Ataxia-telangiectasia mutated (ATM) is a large protein kinase with a central role in the cellular response to DNA double-strand breaks (DSBs) and related genotoxic stress. ATM, which belongs to the phosphatidylinositol 3-kinase-like protein kinase (PIKK) family, is essential for the sensing of DSBs during the cell cycle. MRN contributes to the localization of ATM to DSBs, and together with double-stranded DNA (dsDNA), it activates ATM as a protein kinase.

As the Nbs1 C-terminal half is unstructured or loosely folded, we made cryo-EM grids using a 28-residue peptide (207 μM) that encompasses the acidic region and FxF/Y motif of human Nbs1 (residues 727–754, hereafter referred to as Nc28) and human ATM (1.2 μM). After focused refinements of the ATM Spiral domain, we built a 10-residue Nbs1 segment (740ADDLFRYNPY749) into the improved density guided by the unambiguous density of the side chains for Phe744 and Tyr746. The Nbs1 peptide adopts an overall extended conformation except for one turn of a 310 helix in the middle (residues Asp742 to Arg745). It binds to a hydrophobic groove between two helical repeats formed by helices sα39 to sα42 (denoted ‘s’ for Spiral domain helices). Phe744 inserts deepest into the hydrophobic groove and makes van der Waals contacts to the side chains of Ser978, Arg981, Cys987, Val1021, Ala1024, Phe1025, Leu1028, and Tyr1034 of ATM. Of the two acidic residues that precede the Leu743-Phe744 pair, Asp741 hydrogen bonds with Ser978 and Arg981, while Asp742 is solvent exposed and uninvolved in ATM contacts. Tyr746 is the last Nbs1 residue that contacts ATM. Its side chain, which is stabilized by intramolecular stacking with Pro748, packs with side chain and backbone groups of Gly1016, Gln1017, and Thr1020 of ATM. The ATM structural elements at the Nbs1 binding site, including the hydrophobic pocket and adjacent cleft, are nearly identical in both the apo and Nc28-bound structures, indicating that Nc28 binding does not induce any noticeable structural rearrangements to this region. Additionally, no significant changes to the structure of the kinase domain were observed when comparing the unbound and Nc28-bound states. F744A and FRY to AAA mutations appeared to disrupt the interaction almost completely, whereas Y746A showed an intermediate effect. These results indicate that Nbs1 Phe744 is central to ATM binding, Tyr746 clearly contributes, while Arg745 makes at most a minor contribution in our assay.

>[2x]MSLVLNDLLICCRQLEHDRATERKKEVEKFKRLIRDPETIKHLDRHSDSKQGKYLNWDAVFRFLQKYIQKETECLRIAKPNVSASTQASRQKKMQEISSLVKYFIKCANRRAPRLKCQELLNYIMDTVKDSSNGAIYGADCSNILLKDILSVRKYWCEISQQQWLELFSVYFRLYLKPSQDVHRVLVARIIHAVTKGCCSQTDGLNSKFLDFFSKAIQCARQEKSSSGLNHILAALTIFLKTLAVNFRIRVCELGDEILPTLLYIWTQHRLNDSLKEVIIELFQLQIYIHHPKGAKTQEKGAYESTKWRSILYNLYDLLVNEISHIGSRGKYSSGFRNIAVKENLIELMADICHQVFNEDTRSLEISQSYTTTQRESSDYSVPCKRKKIELGWEVIKDHLQKSQNDFDLVPWLQIATQLISKYPASLPNCELSPLLMILSQLLPQQRHGERTPYVLRCLTEVALCQDKRSNLESSQKSDLLKLWNKIWCITFRGISSEQIQAENFGLLGAIIQGSLVEVDREFWKLFTGSACRPSCPAVCCLTLALTTSIVPGTVKMGIEQNMCEVNRSFSLKESIMKWLLFYQLEGDLENSTEVPPILHSNFPHLVLEKILVSLTMKNCKAAMNFFQSVPECEHHQKDKEELSFSEVEELFLQTTFDKMDFLTIVRECGIEKHQSSIGFSVHQNLKESLDRCLLGLSEQLLNNYSSEITNSETLVRCSRLLVGVLGCYCYMGVIAEEEAYKSELFQKAKSLMQCAGESITLFKNKTNEEFRIGSLRNMMQLCTRCLSNCTKKSPNKIASGFFLRLLTSKLMNDIADICKSLASFIKKPFDRGEVESMEDDTNGNLMEVEDQSSMNLFNDYPDSSVSDANEPGESQSTIGAINPLAEEYLSKQDLLFLDMLKFLCLCVTTAQTNTVSFRAADIRRKLLMLIDSSTLEPTKSLHLHMYLMLLKELPGEEYPLPMEDVLELLKPLSNVCSLYRRDQDVCKTILNHVLHVVKNLGQSNMDSENTRDAQGQFLTVIGAFWHLTKERKYIFSVRMALVNCLKTLLEADPYSKWAILNVMGKDFPVNEVFTQFLADNHHQVRMLAAESINRLFQDTKGDSSRLLKALPLKLQQTAFENAYLKAQEGMREMSHSAENPETLDEIYNRKSVLLTLIAVVLSCSPICEKQALFALCKSVKENGLEPHLVKKVLEKVSETFGYRRLEDFMASHLDYLVLEWLNLQDTEYNLSSFPFILLNYTNIEDFYRSCYKVLIPHLVIRSHFDEVKSIANQIQEDWKSLLTDCFPKILVNILPYFAYEGTRDSGMAQQRETATKVYDMLKSENLLGKQIDHLFISNLPEIVVELLMTLHEPANSSASQSTDLCDFSGDLDPAPNPPHFPSHVIKATFAYISNCHKTKLKSILEILSKSPDSYQKILLAICEQAAETNNVYKKHRILKIYHLFVSLLLKDIKSGLGGAWAFVLRDVIYTLIHYINQRPSCIMDVSLRSFSLCCDLLSQVCQTAVTYCKDALENHLHVIVGTLIPLVYEQVEVQKQVLDLLKYLVIDNKDNENLYITIKLLDPFPDHVVFKDLRITQQKIKYSRGPFSLLEEINHFLSVSVYDALPLTRLEGLKDLRRQLELHKDQMVDIMRASQDNPQDGIMVKLVVNLLQLSKMAINHTGEKEVLEAVGSCLGEVGPIDFSTIAIQHSKDASYTKALKLFEDKELQWTFIMLTYLNNTLVEDCVKVRSAAVTCLKNILATKTGHSFWEIYKMTTDPMLAYLQPFRTSRKKFLEVPRFDKENPFEGLDDINLWIPLSENHDIWIKTLTCAFLDSGGTKCEILQLLKPMCEVKTDFCQTVLPYLIHDILLQDTNESWRNLLSTHVQGFFTSCLRHFSQTSRSTTPANLDSESEHFFRCCLDKKSQRTMLAVVDYMRRQKRPSSGTIFNDAFWLDLNYLEVAKVAQSCAAHFTALLYAEIYADKKSMDDQEKRSLAFEEGSQSTTISSLSEKSKEETGISLQDLLLEIYRSIGEPDSLYGCGGGKMLQPITRLRTYEHEAMWGKALVTYDLETAIPSSTRQAGIIQALQNLGLCHILSVYLKGLDYENKDWCPELEELHYQAAWRNMQWDHCTSVSKEVEGTSYHESLYNALQSLRDREFSTFYESLKYARVKEVEEMCKRSLESVYSLYPTLSRLQAIGELESIGELFSRSVTHRQLSEVYIKWQKHSQLLKDSDFSFQEPIMALRTVILEILMEKEMDNSQRECIKDILTKHLVELSILARTFKNTQLPERAIFQIKQYNSVSCGVSEWQLEEAQVFWAKKEQSLALSILKQMIKKLDASCAANNPSLKLTYTECLRVCGNWLAETCLENPAVIMQTYLEKAVEVAGNYDGESSDELRNGKMKAFLSLARFSDTQYQRIENYMKSSEFENKQALLKRAKEEVGLLREHKIQTNRYTVKVQRELELDELALRALKEDRKRFLCKAVENYINCLLSGEEHDMWVFRLCSLWLENSGVSEVNGMMKRDGMKIPTYKFLPLMYQLAARMGTKMMGGLGFHEVLNNLISRISMDHPHHTLFIILALANANRDEFLTKPEVARRSRITKNVPKQSSQLDEDRTEAANRIICTIRSRRPQMVRSVEALCDAYIILANLDATQWKTQRKGINIPADQPITKLKNLEDVVVPTMEIKVDHTGEYGNLVTIQSFKAEFRLAGGVNLPKIIDCVGSDGKERRQLVKGRDDLRQDAVMQQVFQMCNTLLQRNTETRKRKLTICTYKVVPLSQRSGVLEWCTGTVPIGEFLVNNEDGAHKRYRPNDFSAFQCQKKMMEVQKKSFEEKYEVFMDVCQNFQPVFRYFCMEKFLDPAIWFEKRLAYTRSVATSSIVGYILGLGDRHVQNILINEQSAELVHIDLGVAFEQGKILPTPETVPFRLTRDIVDGMGITGVEGVFRRCCEKTMEVMRNSQETLLTIVEVLLYDPLFDWTMNPLKALYLQQRPEDETELHPTLNADDQECKRNLSDIDQSFNKVAERVLMRLQEKLKGVEEGTVLSVGGQVNLLIQQAIDPKNLSRLFPGWKAWV;>[2x]MEVQNQHAKEESLADDLFRYNPYLKRRR>[2x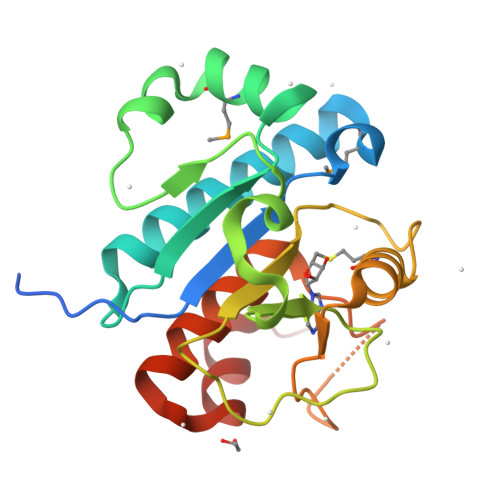]GPNSDGHDRKRVRRDVVHSTLRLIIDCSFDHLMVLKDIKKLHKQIQRCYAENRRALHPVQFYLTSHGGQLKKNMDENDKGWVNWKDIHIKPEHYSELIKKEDLIYLTSDSPNILKELDESKAYVIGGLVDHNHHKGLTYKQASDYGINHAQLPLGNFVKMNSRKVLAVNHVFEIILEYLETRDWQEAFFTILPQRKG> MTTVGFDVAARLGTLLTAMVTPFSGDGSLDTATAARLANHLVDQGCDGLVVSGTTGESPTTTDGEKIELLRAVLEAVGDRARVIAGAGTYDTAHSIRLAKACAAEGAHGLLVVTPYYSKPPQRGLQAHFTAVADATELPMLLYDIPGRSAVPIEPDTIRALASHPNIVGVKDAKADLHSGAQIMADTGLAYYSGDDALNLPWLAMGATGFISVIAHLAAGQLRELLSAFGSGDIATARKINIAVAPLCNAMSRLGGVT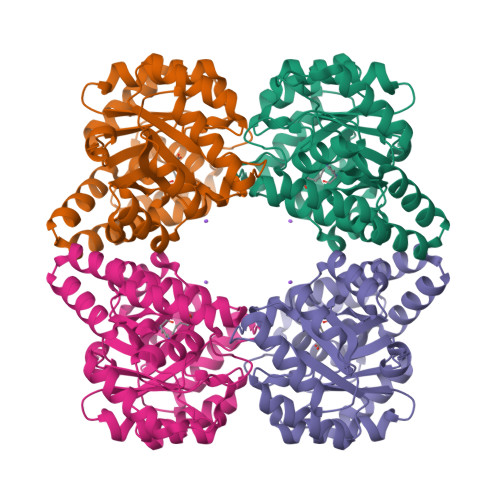LSKAGLRLQGIDVGDPRLPQVAATPEQIDALAADMRAASVLR>[2x]AMVLTPEEKDMIGEIGNIAMGSAATTLSMILGRDIHITVPTVREEKMKNVKSDFSGEQVVVSVEYTEGLEGLNVLVLDKKLVAVIADLMMGGSGEVETEELDEIKLS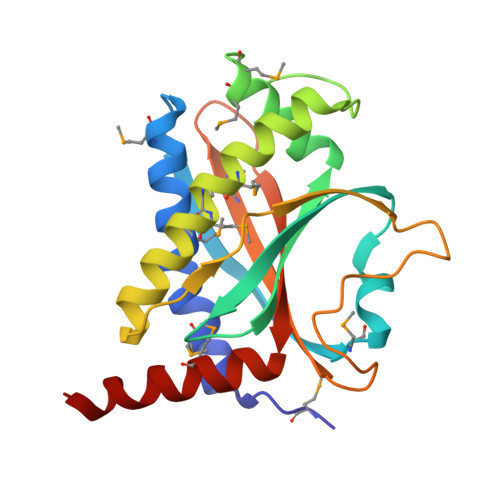AVGEAMNQMMGSAATSLSELLGITINISPPKVEILNFDDPNTQFPPVTDNPEKDVAVVEFEMEIEGLPKSKFYQVISADLVKKMYEYFTKKQSEA> MRCIGMSNRDFVEGVSGGSWVDIVLEHGSCVTTMAKNKPTLDFELIKTEAKQPATLRKYCIEAKLTNTTTESRCPTQGEPSLNEEQDKRFVCKHSMVDRGWGNGCDLFGKGGIVTCAMFRCKKNMEGKVVQPENLEYTIVITPHSGEEHAVGNDTGKHGKEIKITPQSSITEAELTGYGTVTMECSPRTGLDFNEMVLLQMENKAWLVHRQWFLDLPLPWLPGADTQGSNWIQKETLVTFKNPHAKKQDVVVLG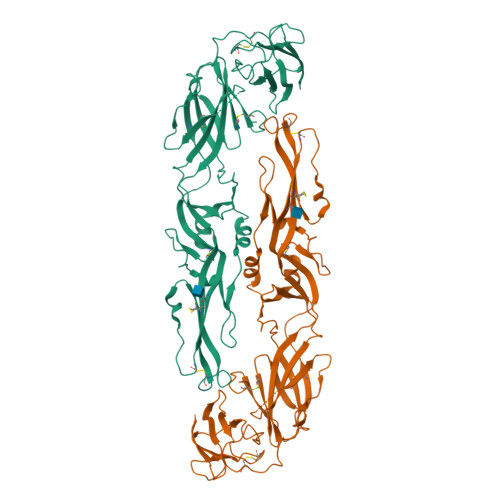SQEGWMHRALTGATEIQMSSGNLLWPGHLKCRLRMDKLQLKGMSYSMCTGKFKVVKEIAETQHGTIVIRVQYEGDGSPCKIPFEIMDLEKRHVLGRLITVNPIVTEKDSPVNIEAEPPFGDSYIIIGVEPGQLKLNWFKKGSSGGSHHHHHHHH> MDSNDLEASFTSRLPPEIVAALKRKSSRDPNSRFPRKLHMLLTYLASNPQLEEEIGLSWISDTEFKMKKKNVALVMGIKLNTLNVNLRDLAFEQLQHDKGGWTQWKRSGFTRNSVFEDPTQNDSPMHHHH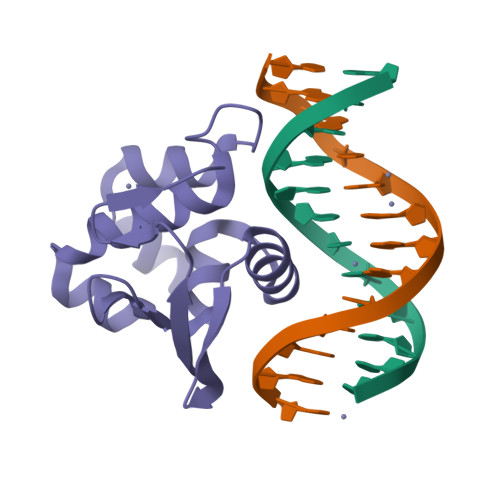H> QELPQMTQQLNSDDMQEQLSATVKFRQILSREHRPPIDVVIQAGVVPRLVEFMRENQPEMLQLEAAWALTNIASGTSAQTKVVVDADAVPLFIQLLYTGSVEVKEQAIWALGNVAGDSTDYRDYVLQCNAMEPILGLFNSNKPSLIRTATWTLSNLCRGKKPQPDWSVVSQALPTLAKLIYSMD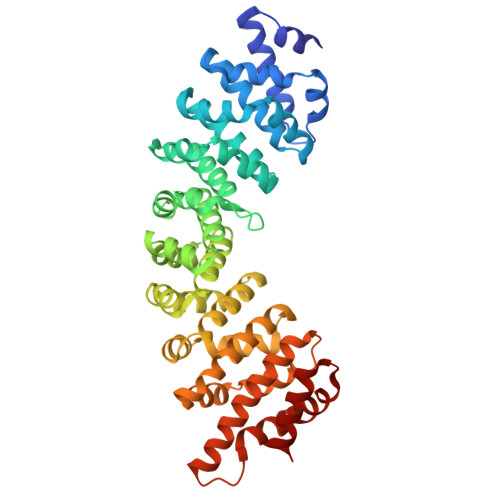TETLVDACWAISYLSDGPQEAIQAVIDVRIPKRLVELLSHESTLVQTPALRAVGNIVTGNDLQTQVVINAGVLPALRLLLSSPKENIKKEACWTISNITAGNTEQIQAVIDANLIPPLVKLLEVAEDKTKKEACWAISNASSGGLQRPDIIRYLVSQGCIKPLCDLLEIADNRIIEVTLDALENILKMGEADKEARGLNINENADFIEKAGGMEKIFNCQQNENDKIYEKAYKIIETYFG>[12x]SFFSFLGEAFDGARDMWRAY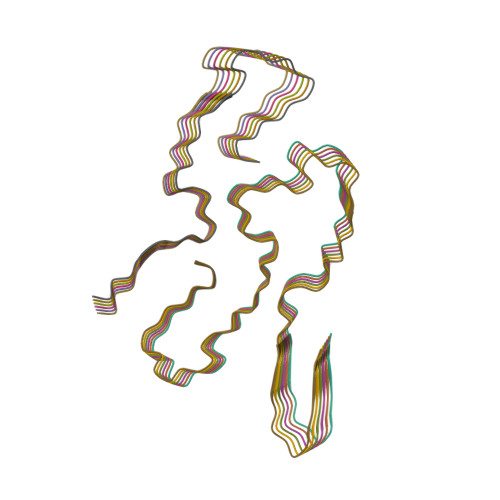SDMREANYIGSDKYFHARGNYDAAKRGPGGVWAAEAISDARENIQRFF>MTDMNILDLFLKASLLVKLIMLILIGFSIASWAIIIQRTRILNAAAREAEAFEDKFWSGIELSRLYQESQGKRDNLTGSEQIFYSGFKEFVRLHRANSHAPEAVVEGASRAMRISMNRELENLETHIPFLGTVGSISPYIGLFGTVWGIMHAFIALGAVKQATLQMVAPGIAEALIATAIGLFAAIPAVMAYNRLNQRVNKLELNYDNFMEEFTAILHRQAFTVSESNKG[5x];>[2x]MGSWSHPQFEKGSSKATEQNDKLKRAIIISAVLHVILFAALIWSSFDENIEASAGGGGGSSIDAVMVDSGAVVEQYKRMQSQESSAKRSDEQRKMKEQQAAEELREKQAAEQERLKQLEKERLAAQEQKKQAEEAAKQAELKQKQAEEAAAKAAADAKAKAEADAKAAEEAAKKAAADAKKKAEAEAAKAAAEAQKKAEAAAAALKKKAEAAEAAAAEARKKAATEAAEKAKAEAEKKAAAEKAAADKKAAAEKAAADKKAAEKAAAEKAAADKKAAAEKAAADKKAAAAKAAAEKAAAAKA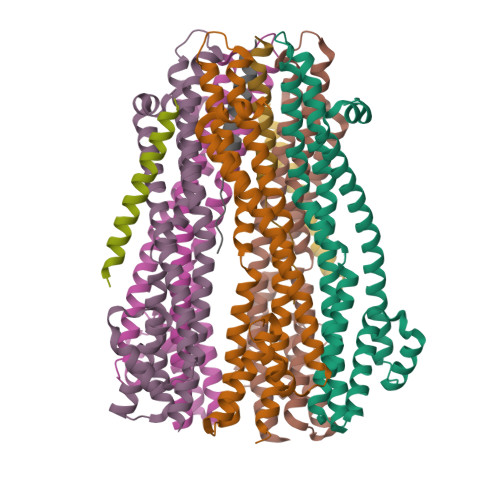AAEADDIFGELSSGKNAPKTGGGAKGNNASPAGSGNTKNNGASGADINNYAGQIKSAIESKFYDASSYAGKTCTLRIKLAPDGMLLDIKPEGGDPALCQAALAAAKLAKIPKPPSQAVYEVFKNAPLDFKP;>[2x]MARARGRGRRDLKSEINIVPLLDVLLVLLLIFMATAPIITQSVEVDLPDATESQAVSSNDNPPVIVEVSGIGQYTVVVEKDRLERLPPEQVVAEVSSRFKANPKTVFLIGGAKDVPYDEIIKALNLLHSAGVKSVGLMTQPI>[4x]MGRENVLPVHNDVYEDFVFTTPYFQPESTFKSVPKLFSDILLGGVEWVYTTSESVLAYDYKLWYLWSGVSNLDESFDMFFNQYWALSLSTSVFQLFYAVILDRYLSVLFQNTPYTNDWFRMMLHSKETALIWLYHPELSWHINGLNQFFTYFYGGILEFVYFDKSNPDMCILVHTLWIHLLILFLIFTGFVTILFSFYGNPNTEENTIDSDYLAASGTVEAEKEITSIDDYLGLVFAIAYVFGVFFYVHGWTSMLSHAVLLLSCYSIIIMFLFILGMPTLLLYDFGIFFLAYLKGAGKYISSVAEMMFDYTACLVFYIRILAQWIRVVLMVVTFISLSHYVSDFDITNSALIGSENQSDSMNELNTNFSMTYYILTVLPGKFIYWIYEILHTFFVVCSQFVAFFAIVFWLFLFLYTFFIIEKHEDFFSKKREERKKKLKELWNLKN;>[12x]MIRNFHSLVKRVPRLALTPFFGFRTSMTLADKKLSTGEASVVLAEKIKGITQQNDITEYGTVISIGDGIARVFGLTKVQAGEMVEFKSGIRGMALNLETDNVGVVVLGNDRDIKEGDVVKRTGAIVDVPIGEAMCGRVFDALGNPIDGLGPLKTTQRARVEIKAPGIIPRQSVRQPMQTGIKCVDSLVPIGRGQRELIIGDRQTGKTAIAIDTILNQKEAFNTGDVKKQLYCIYVAVGQKRSTIANLVSILKQHDCMKFTIVVCATASDAAPLQFLAPYSGCAIGEFFRDNGKHALIIYDDLSKQAVAYRQMSLLLRRPPGREAYPGDVFYLHSRLLERAAKMNDSLGGGSLTALPVIETQAGDVSAYIPTNVISITDGQIFLETELFYKGIRPAINVGLSVSRVGSAAQIKAMKKIAGNLKLTLATYRELAAFSQFGSDLDAKTQQQLNTGERLVEMLKQNQYTPMKVEEQVCIIFAGVKGFLDALVTSEVLKFEKKFLEHVRTNHSALLKRIRDSGDLSEVDTNELNTIIPLFIQEGGFKLKAQ;>MHSTLRVFTKNNCLSFTNMNRFSTAAQVAQANYSKFRADYSASVAAFQQRIKTIEKENTGSMKKPMAKAYEHPYNSEHHPLNFSAVKIAETFHDFIGPEQVSPHYESFAMSRKFLLTFWGGFFVLNFGMATVDLNWIMKSTYIPWIFWFQLMYFYVEGKNSMFMPLLQRFYRRAAANEIFTMEAFYHENIENKLRNLMRITKGQLEYWDIHTSYGEIRADSINNFLANEYLRLQSHITSRALNILKQAQAYETMNQAALLQKLIDDATSAIDNALKGDKKAEVLARSLDSAIDGLSKGYMDYQNDPLLPLILSSIEANVKKITTLSAQEQANLIGLTAEQLKSIKENDVRARKEFLESQPKLDNNLKNIESVKKILATWGK[4x];>MITILDYLFLLDLNDDLTRKAVFEQVIIFIFIYCTMNFLAWSTVVELIWPTHFFNRRHSSSQEFIRFRTYTEVLLKISAYNDFFYVLNNYYYNQKLILKN[4x];>[4x]MSMLAKIAKNVVKTQALKNTTAAQTPSFQAPGNQDKILKWISTLSNKATTGESRSYCTQLSSLVSFYNKQHVEQIPTIDFNEWKSVISTQGLVDKVKENYESLIKEQYNTDAISKQISSASSKALDDIENELSFHAAIWLNAYADYTMFLFELEEYNDPNDYLMHENFDFFRGLETELEELTETHNYIPGAKDDVNLRGYLATQFAWGKKVISFYRHPADDFKCAKATKNMLGR;>[12x]MLSKALQRGIARAFSTTAKKEAPKTVKANGQVSQVIGAVVDVQFEGELPQILNALEVQGTQHRLVLEVAQHLGDSRVRTIAMDSTEGLVRGQPVVDTGLPISVPVGPGTLGRIMNVIGEPIDQRGPIKAAKLYPIHRDAPSFTDQATSAEILVTGIKVVDLLAPYARGGKIGLFGGAGVGKTVLIQELINNVAKHHGGYSVFAGVGERTREGNDLYHEMMDSKVISVKEGESRCALIFGQMNEPPGARARVGLTGLTVAEYFRDEEGKDVLLFVDNIFRFTQACSEVSALLGRIPSAVGYQPTLATDLGALQERITTTQKGSITSVQAIYVPADDLTDPAPATTFAHLDATTVLNRGLTELGIYPAVDPLDSTSRMLDPITIGEEHYTVARGVQKLLQDYKSLQDIIAILGVDDLSEEDKLVVARARKVQKFLSQPFFMSEVFSGIPGRFVNLKQNIASFKALLEGAGDEYPESCFYMKGDLEESLAAGRADALKSK;>[4x]MIHCLRNIRTVSALQSKISYNLGGGNKRKKTSGDLDNYDVLFVGANLGGICSNHFDKDTHGKYKCFVSFDQPINQIYSVRIPYEQQRVRKSEYIHFSKKSINQFTPSEMLAVKEILPEQNAVVLSSGRRIGYNQLVLATGLKHDFSQIKGFYEALEHPEHPVYANRDPETWRSAQHKYSKYISNFKSGDGYFCIPEYPYAGEVECFNFFVSDEVWKWAQHHGALSPKHTFTIVNANEKFVHYCDSADAFIKERLEKRGIRVEYNTKLLEVHQDGQKATFINTKTGEKSVRDYNNLYSIVPSKRQEFLDKAGLTNGNGLLNVDHQTLQHKKYKNIFGLGDAADLPTTKTFWAGWYQIAVVRNNVKRNLQGQTLNAHYDGFSKVPLFTGHQTLTYVAHSYGGVGNWQHLKHNNGGILAWMRYRSWAKGMAKKFQDFYNGARLGPPYHKVLKSFPELPGSPESQQSSGISKYFPTKTENKAAH;>MSLHEKMQTDYLWVKDHSQADSWAKARTHGYNYIAHTVPNKKERYEMIWRSMGKSTDWELEKFRLGKKFPDRGNKRRWFKNLFRLIKNPMGYIFWKTYKARLAKPSLIVTSMFIGFTLGFIKLKAQSIAYSKKQYATLRAGKNIEGSGQVHFGYHDQKWGMPAIPMFQLMYYELPGNSIVVNPCRNQNYRLYFEMRKKLGILPA[4x];>[4x]MINRSTAFISKNLRQANLTQSSLAMKTQYNQMGFSSDNPYNKRWEYKWKHSYYTYPRDYEHTEVRKPQDSKDVPPIYFAYYKDFVDRWLPGMNMWWQRRHRIFDKFNVYFLPGMSLFFYQFADLALGFKIMAAFPLFLAYTRIRDKTLDPDFKETYLRDMIYQNPEITKYFNEETIHVLDYEFEYLPGYLCPEKFPEYQNKTWQFFNTDTAQAEGFFKFGDVESGATMTLKFKTMPIPGKFRYQVGEPFYFYDLRAEIKCDGVYKEVVLVDEKESLKKIRPFLFLI;>[4x]MQVIRKHLAQKGLFNPFLFNRFSTQQDITSVPGDKPPAIEDSIHGKYAGVLFSSASSNKSLNKVAEDMKYFNQLYKESEVFKSFLNNVSLKRNQQRDIISALGKTNFNPATNNLLETLIENKRLDSLPKIAEKYMDYYRILNKQESITIISAQELTAAEKQKVEQGLKKGNANVQFTVVYQVDPAILGGLQMYSGNNFLDCSLLSRVNKLKTEIAKISF;>[4x]MQQRKKIYLRQKRKIYIQLKNKEKKKNNQFIQKREKMGYKIRNKSIFWTRAGWKNNWHPKNFNAPRPSYGEFTMGIRCRNDHHSFLRYVQTYRNMSRHCKQYFLGDKQLEETFILGLRSLFLVPYDSQCLTDQIKHGGERRFVDQLDRDFELISYNTHPYQLFTYTVRNEHLAWKNEQYEKIQKGEKTFEQELLDYLDEQVLAEKAKLRDGQNFSIERMTEIALHVFRKARAGKVRPAQDVRGPDGNVNDFLEQRRPFEHPNPTGVTH;>[40x]MLLVKAVKVLVMGGCMLPIAFGALGTGVLFAGFNVALSRNPEETESLFNNTLMGFALIETFIFMSIGLGFFVLFAA;>MNPIQKAWLKILEPVSYVINEKMAKRTGIIGKLGRFFAIGPREYGVHPINRMFIFMNRKYMAFQAVALHRYSFVKSLTHNGFHMLRVFRHFAFVLPATVLAGLGLFVYWGDDNKCYSPDRFPYLKKRAGDMALPLNSLNQRTSAHYIEINAIYGAEMMKRYHKVWENIIEERSKATDQEKKTRYAHPSYQYSPLPVVSIPNVLNPLNLQ[4x];>MSENKAPGQIYAYDIHNTHYPYVNIKQDSQTQLLASFRRSIASINPFSYRQVPSQDRAAFGLRWGNAWYAPNPYPNGIHFDRVFPTHYDPLAETNRTKANLQLIKYAPGNYSTLVVTSEKLPRPCIRTIQNYRRCQMVNGTEKCNSEAQDILAICPNWALDHMKEKVRFYTKALAINNQTYIRAMQVEEYNQGRTVADVAPKTWIHGTRQHLRPDTMWADDRYTNITQTEINEAIKRVEARKAREHEKKPVEQANVNANTGEQPVRVEKSLYP[4x];>MWYKYFSKQSWNLRVWRKANLKYNQDDFGMTQPKYIARFGDFRFRLVRTEGALRGCMFFVGFGCFSIINYLYGRYGYIINESSQKRAAQDLLDNDMAADKILFKNRVGAPTRPLRSLDDMMAFLSGSATYDQLADYASYNHAMDVNQDQQAGLDSWMSEKDKNMVKYYQRSLGKKVEGI[4x];>[4x]MPVKEGQAKLWFSTKEEADAYDDKMISNIELKSQDYEDENFSPVFNRKTQEYFLEPSEKFKSDFAELLRPLRSLSFNQVVDRYVLIPPNHTFYRNWTYEKFLGGFGLSYLILRELPLRNFYARVFVMYAFAAKVLDHLGNPFPFSGHGQIVAAADRWNHWDVRCYDNVMKALKYIRIPTVQNNIPEATRWYGRQPGHLLRADTYWIPNLVSQRFAKHQPAHWDGTQNMPIFRLADPKHKDSYMVQFR;>MDNYFTAITLLGLRDQNLPPFKDARLQRYKSIKKMIDLIETTTKLAPPMPVELFMLNPTDPEWDDDMTYPTITHATALYKSSALAGNLFLYAYNYNNFTANIRLRTMRYLFPVVSLAIFGNIYWDYRSQLVKVNLFDEYIQARAQELVKQNEYLLEHEDVKRYVWWYEDLKETLARVHRQANNHKACDFKDSEIILQDFIRRYTNPKDNLPIKFHPQGQTF[4x];>MEGFIQNKRKKEKEGEEEEESKEKRKQINQLNKQKQEEEKIYQQKKDQKRKKYLYQRKEMTIFAETWEASEYQYRNKANLKTLPVNHLGKLAELKFDFVEYKAHQLIACHLYERMTIHCMNQYGLFKDFYRPECLDAQYYFKTCVELNAAYGIQKKFFPEHFVGSPYARPVPQFQQLGL[4x];>[4x]MKQKINKLLKNKGVQDKYKYLSKLILLDQEIKGKIKRKNKKEKQKRKNKLILEEMQNTTNIVHVPVHMGHTHYFDYIDSFPKLKEGPTLEENHITNQKILREQLISGQQGLEQNLCLRNCFKLSQKRYIEFCLDRKCGGADFQRAATILGYTKN;>MSNIFLELQDGDKTVYTHTSLIEESKQEQIQAIYDKVPQWTNGGRFLGFWLSMEAVNRVQSVAKLPIYYRAGIVATSTLLGGLVSSLVFWKSGNENQVAKLANGAPVYLKKWEVPELSKLYFFLDDDNNFKPSLNHHAVTQGRQYYKIYQHN[4x];>MFRNILSLVTKPSKLSQKTFYNFAAAKNEVQVSKKQQQAGAKRDLTQYVEGQIVNRNQLTLKKQEDIEQYVLKLVRGYFRTTNKQGLNINSVLQDHGLDEFDSIELAMQVEEDLGYVISAETIPVLNKVKHFVNYINHVEQFKAENGKAPIA[4x];>MSQDPKIVNPQLWPNPNKLRFADLYKYQGVEMKKINDSIKNYKAAKFYIGGILGGCLVFKFFIDAAVDKYIFGENGNGGKFLEMQTINSNYDYYYNRQFQRMRYLTEDPAGDDPLQKTKDEHLVDLGFIPKVFGANVEVRKRAPHDKYL[4x];>[4x]MNSLSSKKANSLVFKSIRNFTLQWGSLAERPMVDRVMSTSTWPVPYYQRLFKAYPIREKKDKMSLLLSDIDIDDTNWYQAKDFLRGSFRGRQIVDYVENNIASNTYILIQQDVANMAKAYVHDICGYIDVANKENVRILSKGDLI;>MFTRFVTQPTLLTQTQRALFSALTKKQKMEVTLRTPYKEYLANFDGFSRITAKTNEASLVIQNKTPASLYVLPPGPLKIRFTSEVKNVSGDFLHTGGWVIVHADNTCEINVMDLFDRKEVRADQFEKGNIQDLDTLAGKYAAKSRKSTVRLFTKATTQ[4x];>MCIEFAFKKAGIPIVRNFLHSTEGVIYGLPQRVQRNLAINYTVKQYKEGKAVSAKTIKTLQEAFPSKGDTK[4x];>[4x]MFGLASKGFINTSLVMVPQMNFGANLKQLKIRMKAIGSIKKITKAMKMVAASKMKAETSRLENGRNFAVGSVQKMLENESYVQKKKSTTAPKSTLLVPITSDKGLCGSVNSSIVREVKRLALNNRSAFGLLPVGEKGSSGLSRPFPDLLKSSIVNIQNVNFPTAAAIAHQVSTQGAGYDQVTLIYNHFKNAISYVVKHQELLPRAQFLNLFKYVTRHEAVEPELEYSKNYFFELYMASSVYNALLNSSASEQASRMNAMENASKNAGEILSKLTLDYNKARQAKITMELIEIISGASIV;>MNRSVNIAKNLIQTYRAMSVQSRFAFSTREEEWLDKRTKSQEKVYFDQEDRKAMKRLLEKLNTTSKFVEDSEYLAPQNLEVENILKRYHINYTQALIDELVDWKTGKN[4x];>MKMEYLQSEEKKDAINKQIHKKEEKEEKEIKIKRKNKVKQRIQIINQIKKYIEAKQQKKQIQSKNQRKYKGRMINTRKQVFKCLWGAQPAYNFSRIINHLRGDPVYQDNTKDVSLRGTFLRGKYDDLPTMIFFTEACDLTANWIPFFTNPQYDILAHRNVWLLNPRNFGNSDRHPSFDLQEMSDDVMRFMYSQKISMATLGGHGIGGKIALAVGCYHAERVTGVFSIDSSPMDQRYHEAFKEFKGYVNALTEINFKTWSDKDVKVFLKENIKDPKWRSIFTNNISKNAKTQSDSFNFEINYLNHNLNFNKADSLGNWAVKNGIYTGRAHFIFPEYSRWVHLATNTLPMHKVCARVKGFGHDIFYVQGDENPLNHWVYDFENYANVVASKLNKFLHSYDGVHALLKDRTEIGNFMIPDRIKSRNDSKHIYGDYSPAHLHHNWRFNHIYEKHDELDKKLNEQ[2x]

The F-type ATP synthase (F1Fo-ATP synthase) is responsible for generating most of the cellular adenosine triphosphate (ATP) from adenosine diphosphate (ADP) and inorganic phosphate through rotary catalysis. In eukaryotes, ATP synthases are found in the inner mitochondrial membrane. The type III ATP synthase was detected in ciliates where it induces tubulation of the cristae membranes. In this study, we present the cryo-EM structures of the type III ATP synthase dimer and tetramer with associated lipids from the model organism Tetrahymena thermophila in complex with the natural inhibitor IF1.

The tetramer was refined to 3.3 Å resolution and the membrane region consisting of interacting Fo subcomplexes was further improved to 3.1 Å resolution upon masked refinement. Two copies of the ATP synthase dimer model were refined into the Fo-tetramer map generating a composite ATP synthase tetramer model. All protein densities could be explained by subunits of the dimer models, and no additional protein moieties appear to be needed to hold the tetramer together. In the tetramer, the ATP synthase dimers are spaced 140 Å center-to-center with an angle of ~11° between dimer axes bringing the Fo-subcomplexes together. In addition, along a perpendicular axis parallel to the membrane plane, the dimers are arranged with a ~3° angle. This angular arrangement induces curvature of the surrounding membrane in a right-handed helical shape, which is also evident from the detergent/membrane density surrounding the ATP synthase tetramer. The protein-protein interactions holding the two dimers together can be classified into two interface types: direct interactions between Fo subunits in the lumen, and interactions mediated by lipids. The analysis of the interface forming the tetramer revealed that the specific N-terminal helical bundle of subunit-a functions as an adaptor for subunit-i/j and ATPTT6 that are positioned to engage in interactions associating two neighboring dimers in a tetramer. By extrapolation, the same interface is available for the addition of multiple dimer modules, all with an angular arrangement represented by the type III ATP synthase tetramer structure. This produces a right-handed helical row with 36 ATP synthase dimers per helical turn, which underpins the organization of the inner mitochondrial membrane into tubular cristae.> PQQKRSSPSEGLCPPGHHISEDGRDCISCKYGQDYSTHWNDLLFCLRCTRCDSGEVELSPCTTTRNTVCQCEEGTFREEDSPEMCRKCRTGCPRGMVKVGDCTPWSDIECVHKESGD;> PQRVAAHITGTRGRSN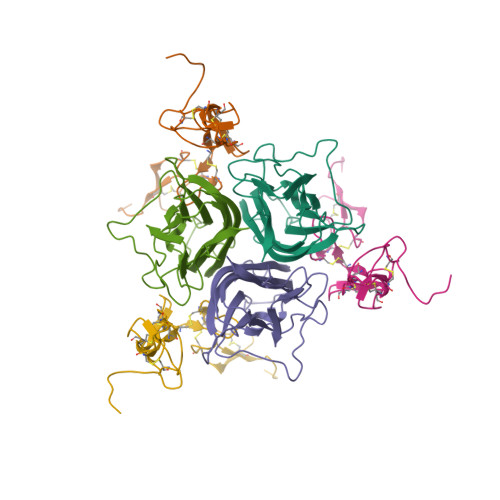TLSSPNSKNEKALGRKINSWESSRSGHSFLSNLHLRNGELVIHEKGFYYIYSQTYFRFQEEIKENTKNDKQMVQYIYKYTSYPDPILLMKSARNSCWSKDAEYGLYSIYQGGIFELKENDRIFVSVTNEHLIDMDHEASFFGAFLVG> MRGSHHHHHHGSENLYFQSGLFDAPGRSQFVPADQAFAFDFQQNQHDLNLTWQIKDGYYLYRKQIRITPEHAKIADVQLPQGVWHEDEFYGKSEI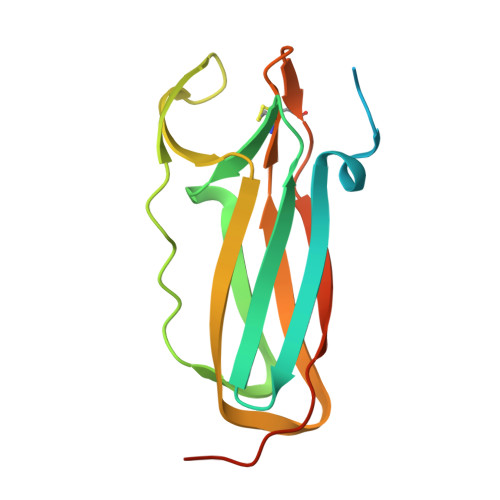YRDRLTLPVTINQASAGATLTVTYQGCADAGFCYPPETKTVPLSEVVANNAAPQPV>AMAQIDLNITCRFAGVFHVEKNGRYSISRTEAADLCKAFNSTLPTMAQMEKALSIGFETCRYGFIEGHVVI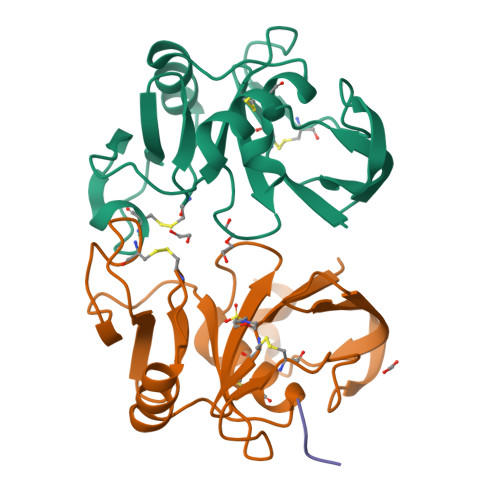PRIHPNSICAANNTGVYILTSNTSQYDTYCFNASAPPEEDCTSVTDLPNAFDGPITITIVNRDGTRYVQKGEYRTNPEDIYP[2x];> AAAV>[4x]GSDASKLSSDYSLPDLINTRKVPNNWQTGEQASLEEGRIVLTSNQNSKG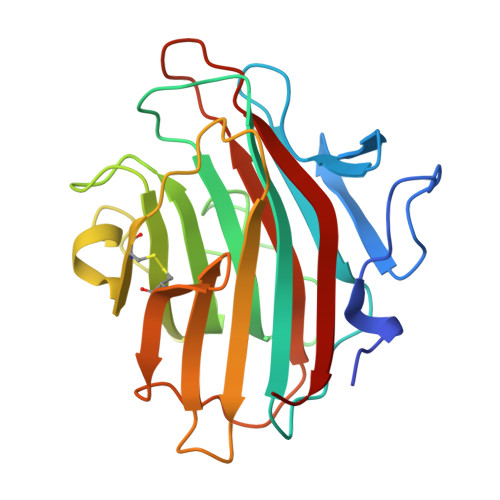SLWLKQGFDLKDSFTMEWTFRSVGYSGQTDGGISFWFVQDSNIPRDKQLYNGPVNYDGLQLLVDNNGPLGPTLRGQLNDGQKPVDKTKIYDQSFASCLMGYQDSSVPSTIRVTYDLEDDNLLKVQVDNKVCFQTRKVRFPSGSYRIGVTAQNGAVNNNAESFEIFKMQFFNGV Bacterial β-lactamases in Gram negative bacteria are primarily responsible for the inactivation of our current β-lactam antibiotics. Penem and penam sulfone β-lactamase inhibitors bearing heterocycle substitutions at the C6 position via a methylidene linkage are two compound classes that inactivate class A β-lactamases by forming a long-lived intermediates. The compounds first form a covalent bond with catalytic S70 concomitant with opening of the β-lactam ring, thus forming an acyl enzyme, followed by opening of the second ring. Despite their similarities, these penem and penam inhibitors undergo different cyclization reactions forming distinct long-lived cyclic inhibitory intermediates.

The SHV-1:SA1-204 structure was determined at 1.53 Å resolution. The initial unbiased omit Fo-Fc map reveals a clear covalent acyl intermediate attached to the catalytic S70 residue with characteristic features including a bicyclic ring and a phenyl tail. In our study of the SHV-1: SA1-204 complex, the carbonyl oxygen of SA1-204 is positioned out of the oxyanion hole and stabilized by side chains of S130 and K234. The bicyclic ring partially occludes the oxyanion hole and makes van der Waals interactions with A237. Importantly, the C3-carboxylate group is noted to form a salt-bridge interaction with R244. Additionally, the sulfone group of SA1-204 interacts with water molecules including a water-mediated interaction with Y105. The phenyl tail of SA1-204 is in van der Waals distance with V216, A217, and L220 and is also close to a Cymal-6 molecule. Compared with apo SHV-1 structure, the most prominent movements of the active site residues are the different rotamer taken by S130 and the outward shift of the V216 containing loop to accommodate the carbonyl oxygen and the C2-methyl group of SA1-204 intermediate. Other potential reasons for the decreased deacylation rate and stability of penam sulfone intermediate include the steric and electrostatic barriers and the spatially increased distance for the approach of the deacylation water to the ester carbonyl. Firstly, in this SHV-1:penam sulfone structure, the deacylation water is positioned 4.07 Å away from the ester carbonyl carbon compared while in the usual acyl intermediate this distance is 2.8 Å.

> MRYIRLCIISLLATLPLAVHASPQPLEQIKLSESQLSGRVGMIEMDLASGRTLTAWRADERFPMMSTFKVVLCGAVLARVDAGDEQLERKIHYRQQDLVDYSPVSEKHLADGMTVGELCAAAITMSDNSAANLLLATVGGPAGLTAFLRQIGDNVTRLDRWETELNEALPGDARDTTTPASMAATLRKLLTSQRLSARSQRQLLQWMVDDRVAGPLIRSVLPAGWFIADKTGAGERGARGIVALLGPNNKAERIVVIYLRDTPASMAERNQQIAGIGAALIEHWQR>[4x]MAKKTGAKYPKSLLSLPLVGSLPFLPRHGHM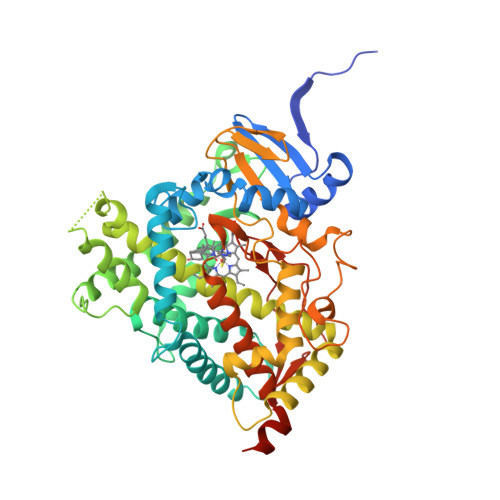HNNFFKLQKKYGPIYSVRMGTKTTVIVGHHQLAKEVLIKKGKDFSGRPQMATLDILSNNRKGIAFADSGAHWQLHRRLAMATFALFKDGDQKLEKIICQEISTLCDMLATHNGQSIDISFPVFVAVTNVISLICFNTSYKNGDPELNVIQNYNEGIIDNLSKDSLVDLVPWLKIFPNKTLEKLKSHVKIRNDLLNKILENYKEKFRSDSITNMLDTLMQAKMNSDNGNAGPDQDSELLSDNHILTTIGDIFGAGVETTTSVVKWTLAFLLHNPQVKKKLYEEIDQNVGFSRTPTISDRNRLLLLEATIREVLRLRPVAPMLIPHKANVDSSIGEFAVDKGTEVIINLWALHHNEKEWHQPDQFMPERFLNPAGTQLISPSVSYLPFGAGPRSCIGEILARQELFLIMAWLLQRFDLEVPDDGQLPSLEGIPKVVFLIDSFKVKIKVRQAWREAQAEGSTHHHH> MQGLKATPGLRASSGRPTLRTARTALVVRAHASQPSSSNHAEQQECSSSGSGVSVNQPSALGRLGKFGLSSALSAFVLVPNFGGFGGNGGNRGGGGGGGGGGGSGGQGQPDGGLPLPLYELAEESSDEKEKQQKDDKRNWKNLVTDSEDLEEKPGERSGTNRCVEIVIEGWPDVGNLPTADELKDLLTVQEGHIFEKQDLLDDRRKLEIQYEDYIAEVEIRTEYVDGKSNHQRVVYKFTPHQFRGINAIDIKGAALMPASEVERICNECLPKQPYMVDIAVMDKVRNRIEQWYQSRGLPFCYVGFFDGMDDGILRANVTEAKIDNVSVRFVRPKLTGDSELEYSVYDEGKVVKADKIIEASGFQRGHHYHVEDGYDAMNSIFACGLLEDINIEPEQDPSDVNKINVKIRCEEVQ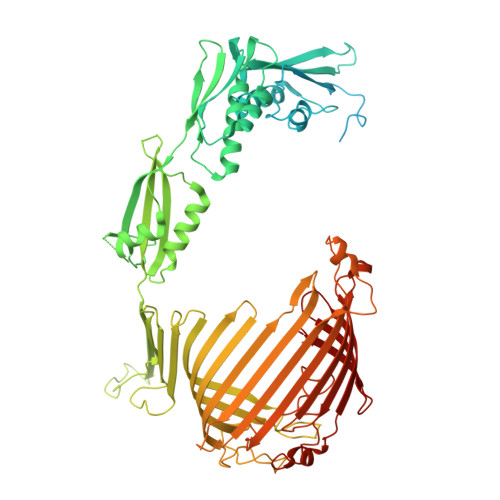PKSMELDLDWSFQLKNGIPSINRQSLIPGGSVEVSHENLFGNSESATLSLSASDWRNPSADLGFSVAYSEPFYKPHTTRNAQLFNTRKTSTIFTPGGESEVPPVFVDRFGLKGWTSQITGQDNKVEHALMLQLVSTLDENGQVVAKGTKVQRGYYADNGPPTTNSGNGRDLSLSYQGFFALDNVRFINGNQLGERMLFQVDQGLNPSISLPGGRKLGLSGGIYNRATASYTKFLEAPFLPKLTTEQLWKERKAPNTVVLHAKAGNALGDVAAYDYFSLGGPYSVRGYSHGEIGAARRFLELATEVRVPLKNYGLPGTAYGFVEYATDLGSGRELNGNPTEYYRKPGRGMSYGLGLKALGACRFEYARDCNAGTGTFLVNFGERF>[2x]GPLGSMKIFL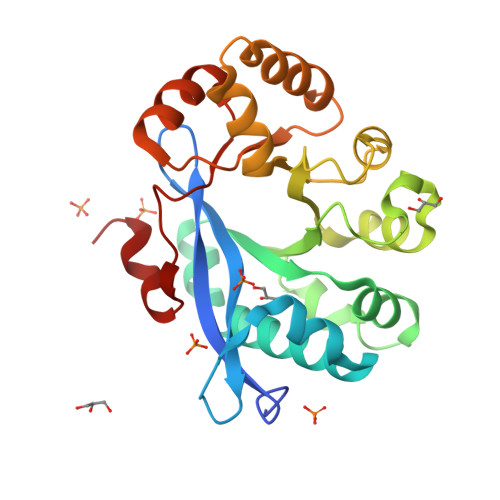ENLYHSDCYFLPIRDNQQVLVGVELITHFSSEDGTVRIPTSRVIAQLTEEQHWQLFSEQLELLKSCQHFFIQHKLFAWLNLTPQVATLLLERDNYAGELLKYPFIELLINENYPHLNEGKDNRGLLSLSQVYPLVLGNLGAGNSTMKAVFDGLFTRVMLDKSFIQQQITHRSFEPFIRAIQAQISPCCNCIIAGGIDTAEILAQITPFDFHALQGCLWPAVPINQITTLVQR(3R,4R,5R)-3,4-dihydroxy-5-({[(1R)-2-hydroxy-1-phenylethyl]amino}methyl)-1-methylpyrrolidin-2-one 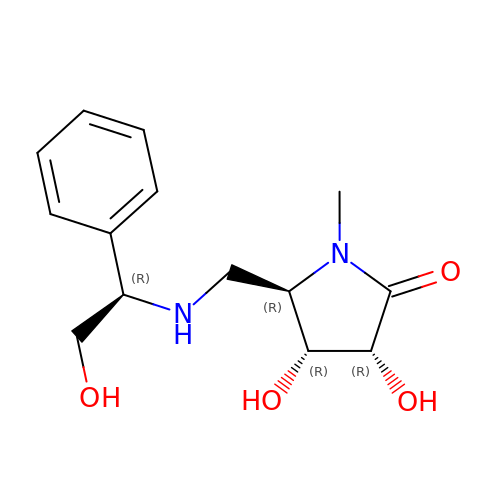| C14 H20 N2 O4 | DNDCXXSXVWBCJF-UMSGYPCISA-N> SLSNKLTLDKLDVKGKRVVMRVDFNVPMKNNQITNNQRIKAAVPSIKFCLDNGAK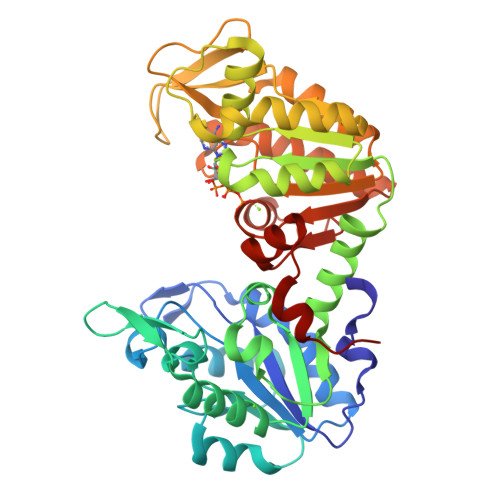SVVLMSHLGRPDGVPMPDKYSLEPVAVELKSLLGKDVLFLKDCVGPEVEKACANPAAGSVILLENLRFHVEEEGKGKDASGNKVKAEPAKIEAFRASLSKLGDVYVNDAFDTAHRAHSSMVGVNLPQKAGGFLMKKELNYFAKALESPERPFLAILGGAKVADKIQLINNMLDKVNEMIIGGGMAFTFLKVLNNMEIGTSLFDEEGAKIVKDLMSKAEKNGVKITLPVDFVTADKFDENAKTGQATVASGIPAGWMGLDCGPESSKKYAEAVTRAKQIVWNGPVGVFEWEAFARGTKALMDEVVKATSRGCITIIGGGDTATCCAKWNTEDKVSHVSTGGGASLELLEGKVLPGVDALSNI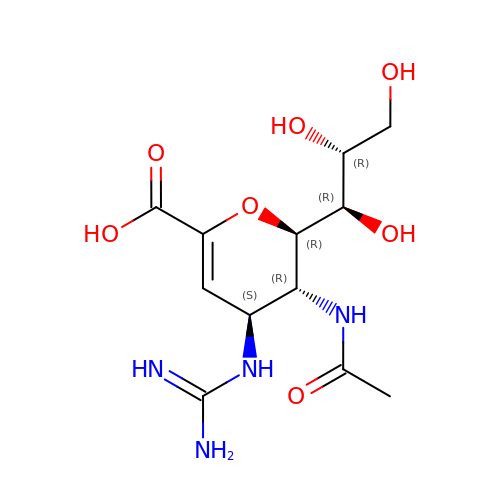ZANAMIVIR | C12 H20 N4 O7 | ARAIBEBZBOPLMB-UFGQHTETSA-N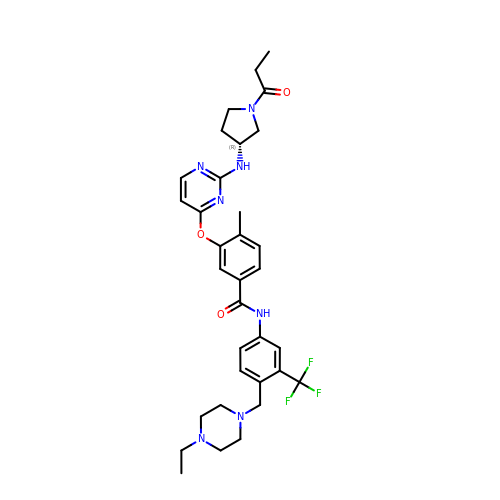~{N}-[4-[(4-ethylpiperazin-1-yl)methyl]-3-(trifluoromethyl)phenyl]-4-methyl-3-[2-[[(3~{R})-1-propanoylpyrrolidin-3-yl]amino]pyrimidin-4-yl]oxy-benzamide | C33 H40 F3 N7 O3 | UGBPGPFLKSJLMW-AREMUKBSSA-N>[2x]MSKPQPIAAANWKCNGSQQS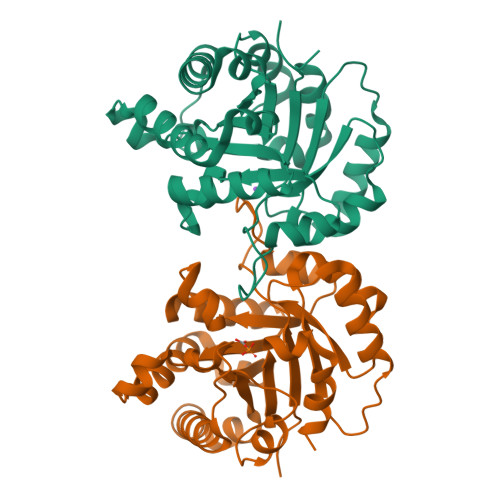LSELIDLFNSTSINHDVQCVVASTFVHLAMTKERLSHPKFVIAAQNAIAKSGAFTGEVSLPILKDFGVNWIVLGHSERRAYYGETNEIVADKVAAAVASGFMVIACIGETLQERESGRTAVVVLTQIAAIAKKLKKADWAKVVIAYEPVWAAGTGKVATPQQAQEAHALIRSWVSSKIGADVAGELRILYGGSVNGKNARTLYQQRDVNGFAVGGASLKPEFVDIIKATQ N-[(1R)-1-(2,4-dichlorophenyl)-2-(1H-1,2,4-triazol-1-yl)ethyl]-4-(5-phenyl-1,3,4-oxadiazol-2-yl)benzamide 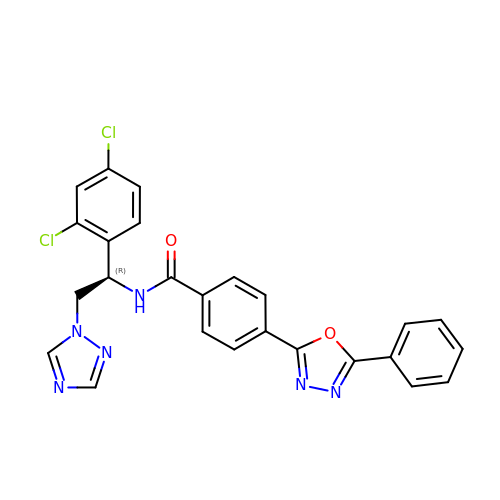| C25 H18 Cl2 N6 O2 | KSMSKLCCSVEWDM-QFIPXVFZSA-N[[(2~{R},3~{S},4~{R},5~{R})-5-(6-aminopurin-9-yl)-3,4-bis(oxidanyl)oxolan-2-yl]methoxy-oxidanyl-phosphoryl] 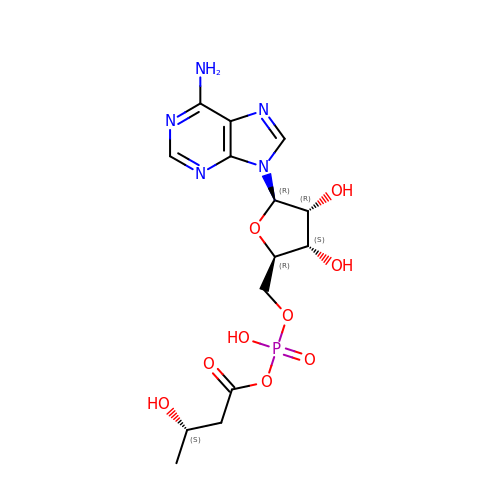(3~{S})-3-oxidanylbutanoate | C14 H20 N5 O9 P | ZNHASVNGLACCHV-LTOLZBHSSA-N CYCLOHEXYL-HEXYL-BETA-D-MALTOSIDE | C24 H44 O11 | 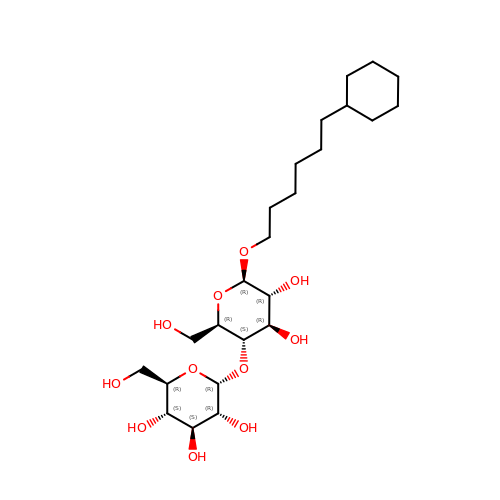WUCWJXGMSXTDAV-QKMCSOCLSA-N Fibronectin (FN)3 and collagen, two essential components of the extracellular matrix, are key players in diverse cellular processes, including adhesion, migration, growth, and differentiation. FN is a high molecular weight multidomain protein composed of three conserved module types (I, II, and III), individual structures of which have been elucidated previously. In vitro, however, 6FnI1–2FnII7–9FnI binds strongly to gelatin, the denatured form of collagen, but not to triple-helical collagen fibrils; 6FnI1–2FnII7–9FnI was thus named the “gelatin-binding domain” (GBD). Collagen binding to the GBD is mediated mostly by the 8–9FnI subfragment, which interacts with sites on D-period 1 (1/10 site) and D-period 4 (3/4 site) of both collagen type I chains.

At a distance of ∼1/10 (D-period 1, peptides AN and CN) or 3/4 (D-period 4, peptides BN and DN) from the N terminus of the triple helix, both chains contain a consensus 9-mer 8–9FnI-binding sequence, in which positions 2 and 9 are occupied by leucine and arginine, respectively. To examine the binding of a collagen 1/10 site, we determined the crystal structure of 8–9FnI in complex with peptide AN. Thus, the molecular basis of this association is the strand extension mechanism commonly used by complexes involving FnI modules, including the high affinity 8–9FnI-BN complex. In-depth comparison of 8–9FnI-AN with 8–9FnI-BN revealed a striking similarity in atomic interactions. We were therefore surprised by NMR titrations, which revealed significantly weaker 8–9FnI binding affinities for the 1/10 sites (KD = 143 μm for AN and 2 mm for CN) compared with their 3/4 counterparts. Just N-terminal of the consensus 9-mer sequence, both high affinity collagen 3/4 sites contain two hydrophobic residues, whereas the weaker 1/10 sites harbor a GTA (AN) or GTO (CN) triplet. This residue triplet makes no contacts with 8–9FnI in the AN or BN complex structure and has poor local electron density. Interestingly, the collagen peptide in both 8–9FnI-AN/BN crystal structures displays a 90° kink just C-terminal to the consensus 8–9FnI-binding sequence, stabilized by hydrophobic interactions involving the Phe92 (AN) or Phe794 (BN) side chain and the peptide main chain. Indeed, when we overlay the 8–9FnI-AN/BN crystal structures onto the SASREF GBD model, the collagen peptides follow the GBD kink, so their C termini would be ideally located to bind to 6FnI1–2FnII7FnI. Thus, we conclude that although the 8–9FnI binding mode is conserved for all four collagen type I sites, residues outside the central consensus 9-mer sequence influence the association strength.

>[2x]DQCIVDDITYNVQDTFHKKHEEGHMLNCTCFGQGRGRWKCDPVDQCQDSETGTFYQIGDSWEKYVHGVRYQCYCYGRGIGEWHCQPLQTYPSS;>GLPGTAGLPGMKGHRGFSGLDGY[2x]> MSEMQGNKIVVDPITRIEGHLRIEVEVEGGKIKNAWSMSTLFRGLEMILKGRDPRDAQHFTQRACGVCTYVHALASVRAVDNCVGVKIPENATLMRNLTMGAQYMHDHLVHFYHLHALDWVNVANALNADPAKAARLANDLSPRKTTTESLKAVQAKVKALVESGQLGIFTNAYFLGGHPAYVLPAEVDLIATAHYLEALRVQVKAARAMAIFGAKNP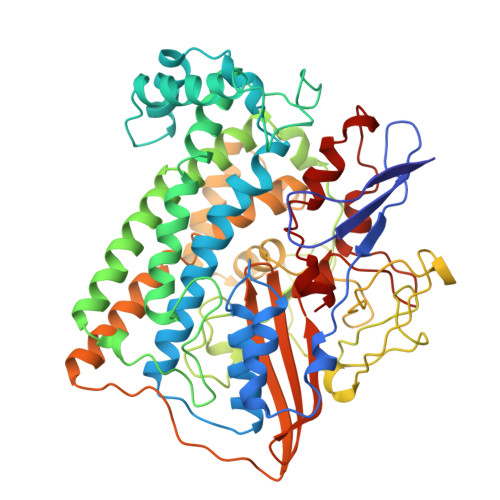HTQFTVVGGCTNYDSLRPERIAEFRKLYKEVREFIEQVYITDLLAVAGFYKNWAGIGKTSNFLTCGEFPTDEYDLNSRYTPQGVIWGNDLSKVDDFNPDLIEEHVKYSWYEGADAHHPYKGVTKPKWTEFHGEDRYSWMKAPRYKGEAFEVGPLASVLVAYAKKHEPTVKAVDLVLKTLGVGPEALFSTLGRTAARGIQCLTAAQEVEVWLDKLEANVKAGKDDLYTDWQYPTESQGVGFVNAPRGMLSHWIVQRGGKIENFQHVVPSTWNLGPRCAERKLSAVEQALIGTPIADPKRPVEILRTVHSYDPCIACGVH> GSTELTPDQQTLLHFIMDSYNKQRMPQEITNKILKEEFSAEENFLILTEMATNHVQVLVEFTKKLPGFQTLDHEDQIALLKGSAVEAMFLRSAEIFNKKLPSGHSDLLEERIRNSGISDEYITPMFSFYKSIGELKMTQEEYALLTAIVILSPDRQYIKDREAVEKLQEPLLDVLQKLCKIHQPENPQHFACLLGRLTELRTFNHHHAEMLMSWRVNDHKFT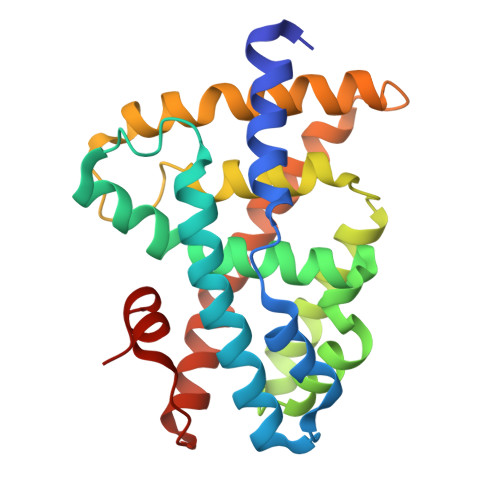PLLCEIWDVQ> MLRRSSAALIRRTPVRHSGGELFVRPKLEEIPPADQCRGFFGPLNDSLKFLRLLDIKWMMNRAVAMRREYLIATPTLFTFIWMFTWKGAVIYFWGDR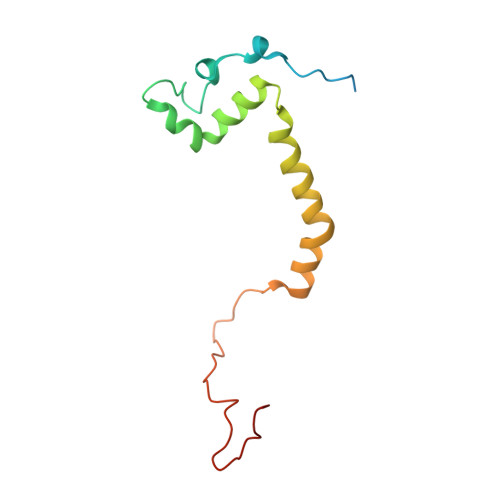APPRRMDWNTEETGRLPLGFKPTPAPL>MSEMDYLENATVIDESALTPEQRLGLKQAEERLERDHIFRLEKRSPEYTNCRYLCKLCLIHIENIQGAHKHIKEKRHKKNILEKQEESELRSLPPPSPAHLAALSVAVIELAKEHGITDDDLRVRQEIVEEMSKVITTFLPECSLRLYGSSLTRFALKSSDVNIDIKFPPKMNHPDLLIKVLGILKKNVLYVDVESDFHAKVPVVVCRDRKSGLLCRVSAGNDMACLTTDLLTALGKIEPVFIPLVLAFRYWAKLCYIDSQTDGGIPSYCFALMVMFFLQQRKPPLLPCLLGSWIEGFDPKRMDDFQLKGIVEEKFVKWECNSSSATKEKHGKSPLALETPNRVSLGQLWLELLKFYTLDFALEEYVICVRIQDILTRENKNWPKRRIAIEDPFSVKRNVARSLNSQLVYEYVVERFRAAYRYFACPQTKGGNKSTVDFKLEHHHHHH[2x]

The terminal uridylyltransferase 4 (TUT4) and/or its homolog TUT7 mono-uridylylate group II pre-let-7, and promote subsequent Dicer processing, since pre-let-7 with a 2-nt 3′-overhang is a good Dicer substrate. Lin28 binding to pre-let-7 competes with the Dicer processing of pre-let-7, recruits TUT4/7 to the Lin28:pre-let-7 complex, and promotes the oligo-uridylylation of pre-let-7 by TUT4/7. The NTD1 in the N-terminal half is inactive since it lacks the catalytic carboxylates for the nucleotidyltransferase activity, while the NTD2 in the C-terminal half is responsible for the nucleotidyltransfer reaction. In this study, we determined the crystal structure of the N-terminal LIM of human TUT4, which consists of ZF and NTD1 (nc-palm and fingers) and is sufficient for the ternary complex formation with Lin28A and pre-let-7.

To obtain the crystal of the LIM, the N-terminal region (residues 1–252) and an internal putative flexible region (residues 579–610) were truncated from the N-terminal half of hTUT4 (residues 1–723), yielding hTUT4_N. The crystal belongs to the space group I212121 and contains two hTUT4_N molecules in the asymmetric unit. The structure was refined to an R factor of 21.1% (Rfree of 23.8%), using reflections up to 2.4 Å resolution. The hTUT4_N protein consists of three domains: zinc finger (ZF: residues 253–343), non-catalytic palm (nc-palm; residues 368–489), and fingers (residues 344–367 and 490–723). The ZF consists of five α-helices (α1–α5) and three β-strands (β1–β3), which compose a large structural domain distinct from other zinc fingers or zinc knuckles, such as the one in the C-terminus of hTUT723. The Cys2His2-type zinc finger motif, in which Cys306, Cys309, His322, and His328 coordinate one zinc ion, forms the core of the ZF. A comparison of the structure of the hTUT4 NTD1 with that of the catalytic domain of hTUT7 revealed that two of the three catalytic carboxylates in hTUT7 are substituted with non-catalytic residues in the NDT1 of hTUT4. As a result, the pocket is totally closed, and the 3′-end of the RNA primer and an incoming nucleotide cannot access the region. The evolutional conservation analysis and electrostatic surface analysis of the overall structure of hTUT4_N revealed that one side of hTUT4_N is highly conserved and positively charged. Altogether, the N-terminal ZF of hTUT4 interacts with the dsRNA region of pre-let-7 and contributes to the stable ternary complex formation with Lin28 and pre-let-7, thus leading to the efficient Lin28-dependent oligo-uridylylation of pre-let-7.Microbial rhodopsins (MRs) are transmembrane light-sensitive proteins, found in Archaea, Bacteria, Eukaryota, and also viruses. MRs are composed of seven transmembrane α-helices (A–G) with the cofactor retinal covalently bound to the lysine residue of helix G via the Schiff base (RSB). Despite this paradigm, the first light-driven Na+ pump KR2 was identified in Krokinobacter eikastus in 20132. KR2 contains a characteristic for all known Na+-pumping rhodopsins (NaRs) set of N112, D116, Q123 residues in the helix C (NDQ motif).

To gather more details about long-distance interactions between the protein core and surface, we solved the structure of pentameric form of KR2-H30A at pH 8.0 at 2.2 Å. Overall, the structure of this mutant is nearly the same as that of the ground state of WT protein (RMSD 0.15 Å). The organization of their inner cytoplasmic, central, and extracellular parts is identical. Surprisingly, in contradiction to the earlier FTIR experiments, Na+ bound at the oligomerization interface of the WT protein is also present in H30A2. However, the region of H30 is altered. Particularly, H30 side chain is replaced by two additional water molecules (wB′ and wB″). Moreover, the H30A mutation leads to appearance of second alternative conformation of Y108, not identified in other structures of KR2 or its variants. It was shown that H30A is more selective to sodium and almost does not pump protons. As the only existing differences in the structures of the WT and the mutant occur near Q78, N81, Y108, H30′ and pIRC2, we suggest that this region is important for cation selectivity, which additionally supports the hypothesis that this region is a part of ion translocation pathway.

>[5x]QELGNANFENFIGATEGFSEIAYQFTSAILTLGYAVMLAGLLYFILTIKNVDKKFQMSNILSAVVMVSAFLLLYAQAQNWTSSFTFNEEVGRYFLDPSGDLFNNGYRYLNWLIDVPMLLFQILFVVSLTTSKFSSVRNQFWFSGAMMIITGYIGQFYEVSNLTAFLVWGAISSAFFFHILWVMKKVINEGKEGISPAGQKILSNIWILFLISWTLYPGAYLMPYLTGVDGFLYSEDGVMARQLVYTIADVSSKVIYGVLLGNLAITLSKNKEL4-amino-7-methyl-2-({5-methyl-1-[(3S)-oxolan-3-yl]-1H-pyrazol-4-yl}amino)-6-[(2R)-2-methylpyrrolidin-1-yl]-7H-pyrrolo[2,3-d]pyrimidine-5-carbonitrile 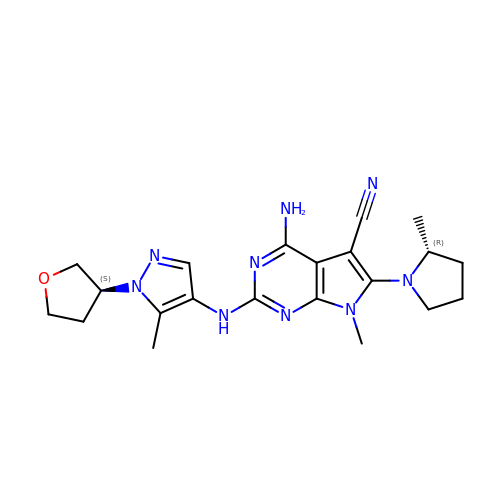| C21 H27 N9 O | QSDVZPULRUJSBC-OCCSQVGLSA-N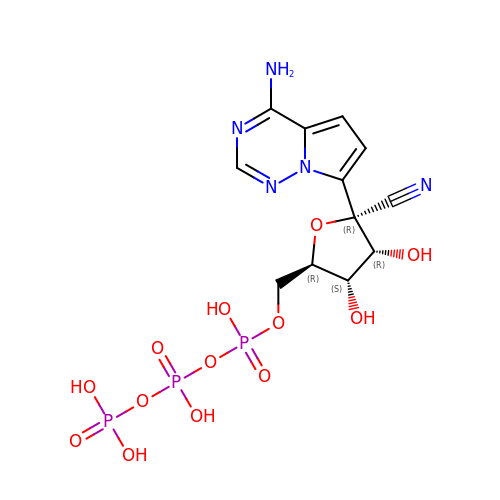[[(2~{R},3~{S},4~{R},5~{R})-5-(4-azanylpyrrolo[2,1-f][1,2,4]triazin-7-yl)-5-cyano-3,4-bis(oxidanyl)oxolan-2-yl]methoxy-oxidanyl-phosphoryl] phosphono hydrogen phosphate | C12 H16 N5 O13 P3 | DFVPCNAMNAPBCX-LTGWCKQJSA-N> MHDFVGFMNKISQINRDLDKYDHTINQVDSLHKRLLTEVNEEQASHLRHSLDNFVAQATDLQFKLKNEIKSAQRDGIHDTNKQAQAENSRQRFLKLIQDYRIVDSNYKEENKEQAKRQYMIIQPEATEDEVEAAISDVGGQQIFSQALLNANRRGEAK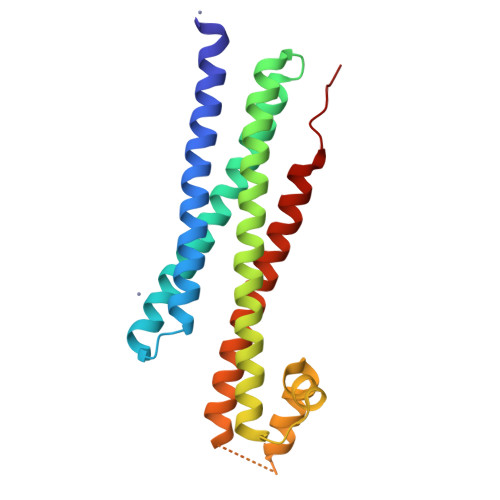TALAEVQARHQELLKLEKSMAELTQLFNDMEELVIEQQ> MGSSHHHHHHSSGLVPRGSHSDEVDAHMESNDSGGVAAKHGFLFQDCVAAYHVTRMLRDKTIRSVRCEVTDDIDIVSDGYIDFVQVKSTGKTRWNISDIVQNSKGADKKTIPCSSILHKSMQCESDLSLGRRYSIVTEEKVNKTLEYLTISPNARLDKPGRQELIDDLNKRTDNFLTDSGISVSDWIDAATWEVFSSLRELELLGIKNIRLASQDLHGVILSSETVAEDIWCRILDTVTRKGEHSRRIHSADDKSYLRPDLLEWFKQRVEDDQSRSGRKIYVKRDLPHILTPFRAPMASVC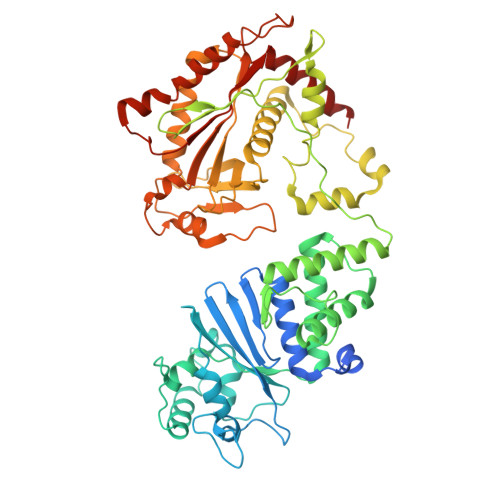AKRKGQVLHQQYSLKKYRYKHIADNVCQWLDEVFLRPKEMSDIHKLTFIEKRERLKNSVFKSLHDVSEFLGRVLLHATIRQHHESQPIPCMLYVEKAGAEKILENVHIVRRDPEGDQLWIGFSELVTDINIAVRLPEIRDQLYEDISDCIDTARKKILDIKDDNYLLRHDIDEILDGSQPFDAHLDRFTFVLFVGYDSNLLTEPETPGFEDDLEKETAVLFEKFAADLIEDSPFANLCIHVFIYPAPSLERLTQLVDEKVREVV> MAKTLKDLQGWEIITTDEQGNIIDGGQKRLRRRGAKTEHYLKRSSDGIKLGRGDSVVMHNEAAGTYSVYMIQELRLNTLNNVVELWALTYLRWFEVNPLAHYRQFNPDANILNRPLNYYNKLFSETANKNELYLTAELAELQLFNFIRVANVMDGSKWEVLKGNVDPERDFTVRYICEPTGEKFVDINIEDVKAYIKKVEPREAQEYLKDLTLPSKKKEIKRGPQKKDKATQTAQISDAETRATDITDNEDGNEDESSDYESPSDIDVSEDMDSGEISADELEEEEDEEEDEDEEEKEARHTNSPRKRGRKIKLGKDDIDASVQPPPKKRGRKPKDPSKPRQMLLISSCRANNTPVIRKFTKKNVARAKKKYTPFSKRFKSIAAIPDLTSLPEFYGNSSELMASRFENKLKTTQKHQIVETIFSKVKKQLNSSYVKEEILKSANFQDYLPARENEFASIYLSAYSAIESDSATTIYVAGTPGVGKTLTVREVVKELLSSSAQREIPDFLYVEINGLKMVKPTDCYETLWNKVSGERLTWAASMESLEFYFKRVPKNKKKTIVVLLDELDAMVTKSQDIMYNFFNWTTYENAKLIVIAVANTMDLPERQLGNKITSRIGFTRIMFTGYTHEELKNIIDLRLKGLNDSFFYVDTKTGNAILIDAAGNDTTVKQTLPEDVRKVRLRMSADAIEIASRKVASVSGDARRALKVCKRAAEIAEKHYMAKHGYGYDGKTVIEDENEEQIYDDEDKDLIESNKAKDDNDDDDDNDGVQTVHITHVMKA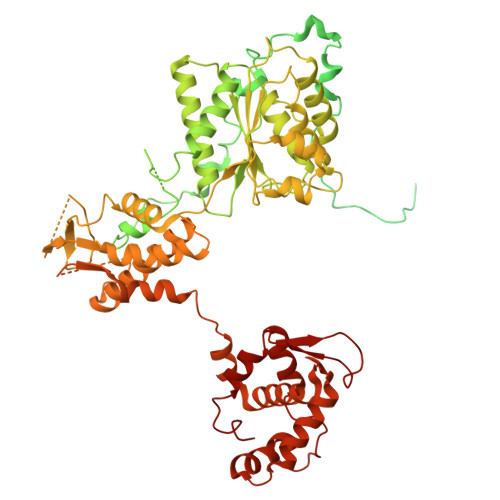LNETLNSHVITFMTRLSFTAKLFIYALLNLMKKNGSQEQELGDIVDEIKLLIEVNGSNKFVMEIAKTLFQQGSDNISEQLRIISWDFVLNQLLDAGILFKQTMKNDRICCVKLNISVEEAKRAMNEDETLRNL>[2x]ACUCGUUUGAGCGAGUAUAAACAGUUGGUUAGGCUCAAAG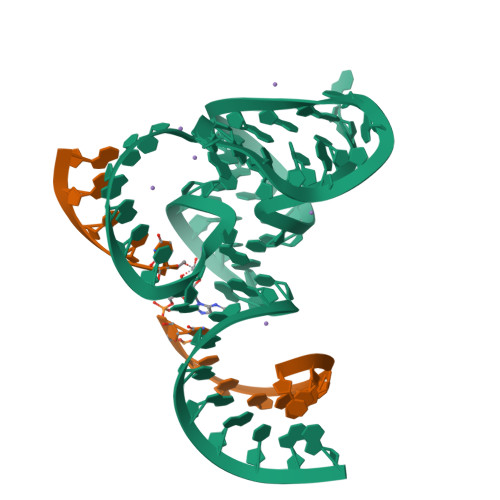CGGAGAGCAG;>UCUGCUCUCXUCCAA[2x]>A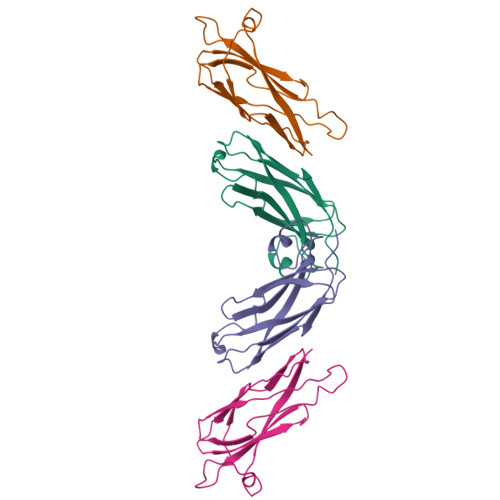QSVPPGDINTQPSQKIVFNAPYDDKHTYHIKITNAGGRRIGWAIKTTNMRRLSVDPPCGVLDPKEKVLMAVSCDTFNAATEDLNNDRITIEWTNTPDGAAKQFRREWFQGDGMVRRKNLPIEYNL[2x]> GSMADEATRRVVSEIPVLKTNAGPRDRELWVQRLKEEYQSLIRYVENNKNADNDWFRLESNKEGTRWFGK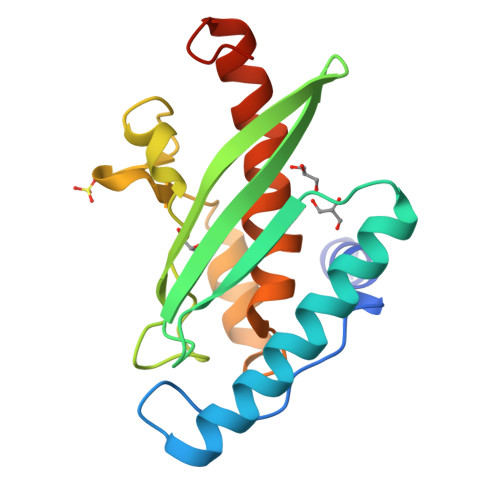CWYIHDLLKYEFDIEFDIPITYPTTAPEIAVPELDGKSAKMYRGGKIELTDHFKPLWARNVPKFGLAHLMALGLGPWLAVEIPDLIQKGVIHHKEKCNQ>LPQMTQQLNSDDMQEQLSATVKFRQILSREHRPPIDVVIQAGVVPRLVEFMRENQPEMLQLEAAWALTNIASGTSAQTKVVVDADAVPLFIQLLYTGSVEVKEQAIWALGNVAGDSTDYRDYVLQCNAMEPILGLFNSNKPSLIRTATWTLSNLCRGKKPQPDWSVVSQALPTLAKLIYSMDTETLVDACWAISYLSDGPQEAIQAVIDVRIPKRLVELLSHESTLVQTPALRAVGNIVTGNDLQTQVVINAGVLPALRLLLSSPKENIKKEACWTISNITAGNTEQIQAVIDANLIPPLVKLLEVAEYKTKKEACWAISNASSGGLQRPDIIRYLVSQGCIKPLCDLLEIADNRIIEVTLDALENILKMGEADKEARGLN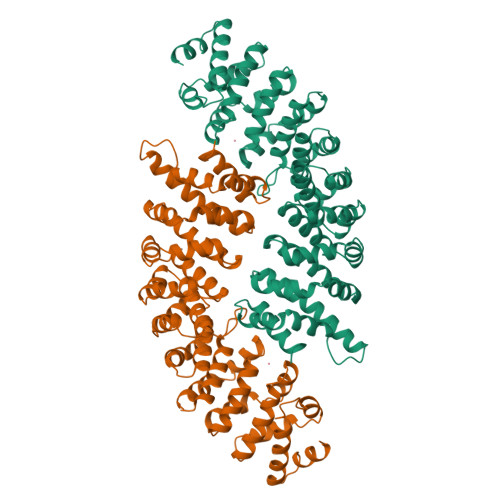INENADFIEKAGGMEKIFNCQQNENDKIYEKAYKIIETYFG[2x]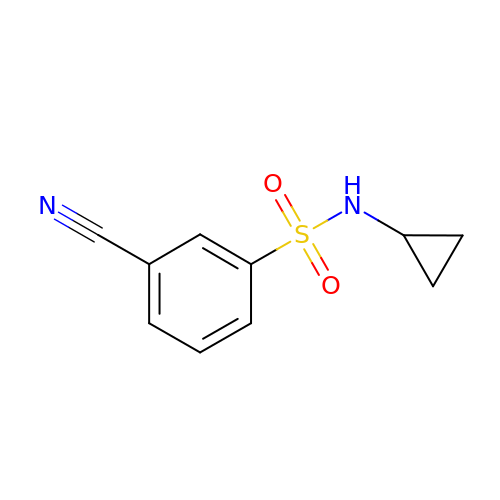3-cyano-~{N}-cyclopropyl-benzenesulfonamide | C10 H10 N2 O2 S | IQBVFUJHLUVSIM-UHFFFAOYSA-N>[12x]SAITSGQELLSQARVLAKYLRDQPEGWLAAHRLMKSVRHDTLHQLPPLSADGRTRIAPPGPDRRASLKRLYLQQNW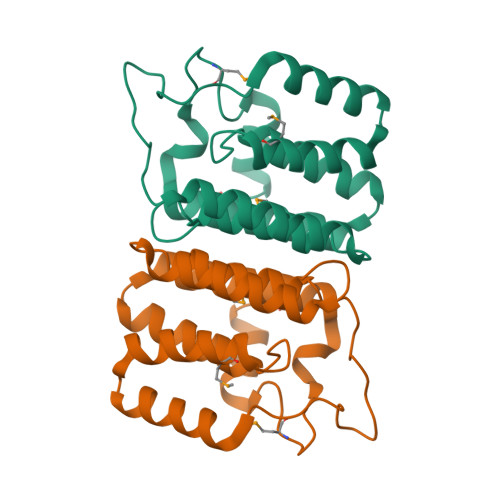LSLLEQCDDMFARGASHLWLDLQWYIHQALLQTGKENYAAIIQYDLKGLLLRLPGLETLAFNDGMPFADDVTLSWIQQQVM>[2x]GSHMHNSNADDAALTTDVVVVGGGPVGLMLAGELRAGGVGALVLEKLVEPVGHDRAGALHIRTVETLDLRGLLDRFLEGTQVAKGLPFAGIFTQGLDFGLVDTRHPYTALVPQSRTEALLAEHAREAGAEIRRGHEVTGLRQDAEAVEVTVAGPSGPYRVRARYAVGCDGGRSTVRRLAGIGFPGTEATVRALIGYVTTPEREVPRRWERTPDGILVLAFPPEGGLGRVVVIEYTGHSPAAD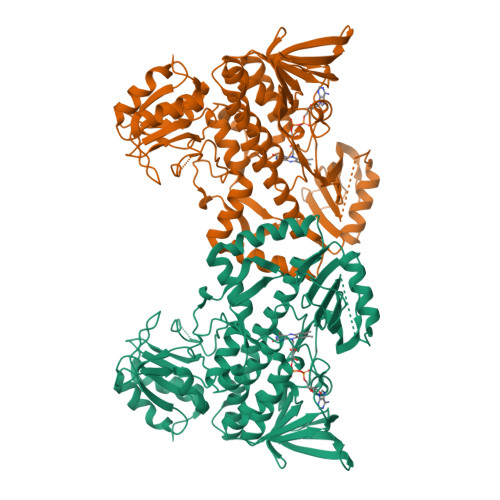EGPVTLEDLGAAVARVRGTPLTLTEPVSWLSRFGDASRQAKRYRSGRVLLAGDAAHVHFPIGGQGLNTGLQDAVNLGWKLAARVRGWGSEELLDTYHDERHPVAERVLLNTRAQLALMRPDEQHTTPLRGFVEELLGTDEVNRYFTGMITGTDVRYATFAPAAPARPHPWAGRFAGGLVLSGPSGEPVPVAELLRSARPLLLDLAGRADLREATRPWSDRVSVVAGEATVEPPAQALLVRPDGYVAWAGSPAATADELRASLARWFGPPANREPVGHQERAGRRGRPLSALKPE> KDGDQCETSPCQNQGKCKDGLGEYTCTCLEGFEG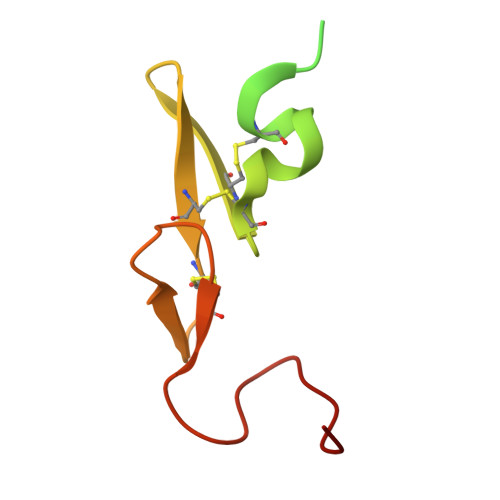KNCELFTRKLCSLDNGDCDQFCHEEQNSVVCSCARGYTLADNGKACIPTGPYPCGKQTLER> IVGGYTCGANTVPYQVSLNSGYHFCGGSLINSQWVVSAAHCYKSGIQVRLGEDNINVVEGNEQFISASKSIVHPSYNSNTLNNDIMLIKLKSAASLNSRVASISLPTSCASAGTQCLISGWGNTKSSGTSYPDVLKCLKAPIL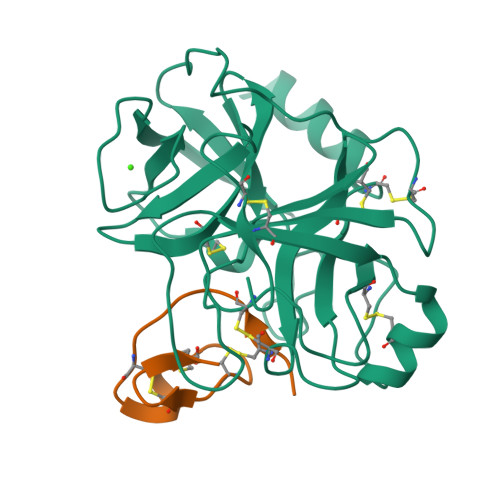SDSSCKSAYPGQITSNMFCAGYLEGGKDSCQGDSGGPVVCSGKLQGIVSWGSGCAQKNKPGVYTKVCNYVSWIKQTIASN;> RICPRIWMECKRDSDCMAECICVMGHCG> MTENAEKFLWGVATSAYQIEGATQEDGRGPSIWDAFAQRPGAIRDGSTGEPACDHYRRYEEDIALMQSLGVRAYRFSVAWPRILPEGRGRINPKGLAFYDRLVDRLLASGITPFLTLYHWDLPLALEERGGWRSRETAFAFAEYAEAVARALADRVPFFATLNEPWCSAFLGHWTGEHAPGLRNLEAALRAAHHLLLGHGLAVEALRAAGARRVGIVLNFAPAYGEDPEAVDVADRYHNRFFLDPILGKGYPESPFRDPPPVPILSRDLELVARPLDFLGVNYYAPVRVAPGTGTLPVRYLPPEGPATAMGWEVYPEGLYHLLKRLGREVPWPLYVTENGAAYPDLWTGEAVVEDPERVAYLEAHVEAALRAREEGVDLRGYF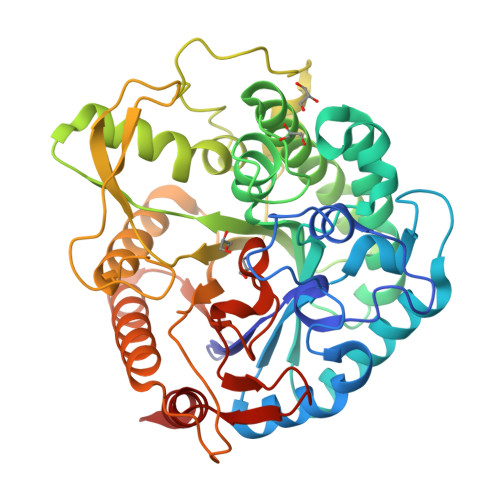VWSLMDNFEWAFGYTRRFGLYYVDFPSQRRIPKRSALWYRERIARAQT Sinigrin | C10 H17 N O9 S2 | 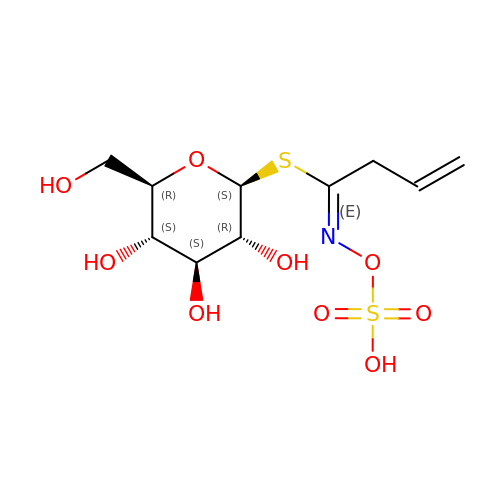PHZOWSSBXJXFOR-PTGZALFTSA-N6-(3-AMINOPROPYL)-4,9-DIMETHYLPYRROLO[3,4-C]CARBAZOLE-1,3(2H,6H)-DIONE | C19 H19 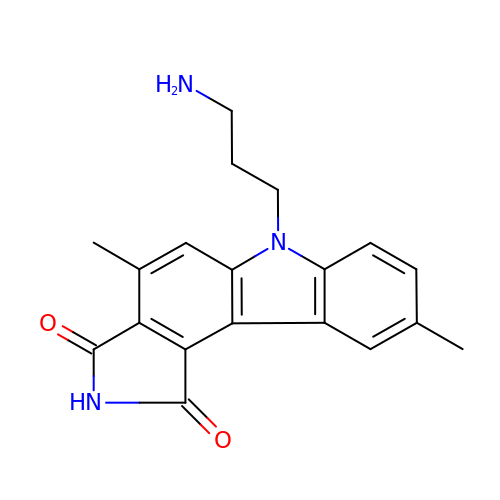N3 O2 | PKPNSCZPIWCHMW-UHFFFAOYSA-N> VVGGMSAEPGAWPWMVSLQIFMYH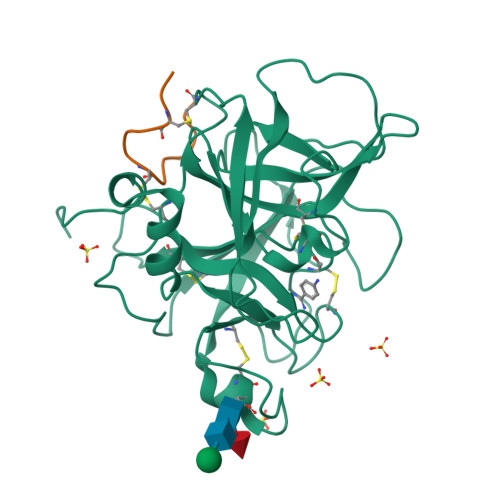NNRRYHTCGGILLNSHWVLTAAHCFKNKKKVTDWRLIFGANEVVWGSNKPVKPPLQERFVEEIIIHEKYVSGLEINDIALIKITPPVPCGPFIGPGCLPQFKAGPPRAPQTCWVTGWGYLKEKGPRTSPTLQEARVALIDLELCNSTRWYNGRIRSTNVCAGYPRGKIDTCQGDSGGPLMCRDRAENTFVVVGITSWGVGCARAKRPGVYTSTWPYLNWIASKIGSNALQMVQLGTPPR;> RDNATCDGPCGLRFRQKLESGMR> GPGSEFMARDYDHLFKLLIIGDSGVGKSSLLLRFADNTFSGSYITTIGVDFKIRTVEINGEKVKLQIWDTAGLERFRTITSTYYRGTHGVIVVYD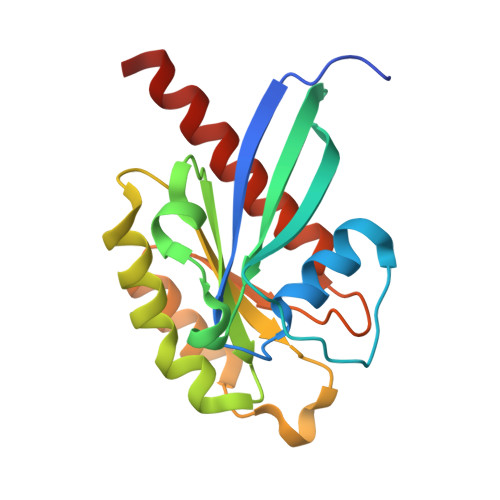VTSAESFVNVKRWLHEINQNCDDVCRILVGNKNDDPERKVVETEDAYKFAGQMGIQLFETSAKENVNVEEMFNCITELVLRAKKDNLAKQQ> GAGC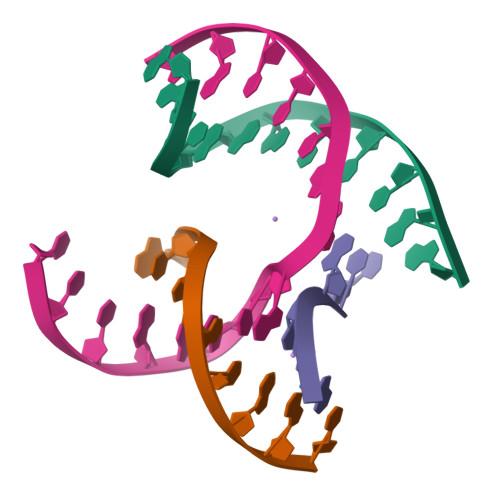AGACTTGA;> CGACACTCA;> TCATCG;> TCTGAGTAGGTCTGC>[6x]MFSKFFIERPVFASVVAIIISLAGAIGLTNLPIEQYPSLTPPTVKVSATYTGADAQTIASTVASPIEDAINGADNMIYMDSTSSSSGTMSLTVYFDIGTDPDQATIDVNNRISAATAKMPDAVKKLGVTVRKTSSTTLAAISMYSSDGSMSAVDVYNYITLNVLDELKRVPGVGDANAIGNRNYSLRIWLKPDLLNKFGITATDVISAVNDQNAQYATGKIGEEPVTQKSPYVYSITMQGRLQNPSEFENIILRTNNDGSFLRLKDVADVEIGSQQYSSQGRLNGNDAVPIMINLQSGANALHTAELVQAKMQELSKNFPKGLTYKIPYDTTKFVIESIKEVVKTFVEALILVIIVMYMFLKNFRATLIPMIAVPVSLLGTFAGLYVLGFSINLLTLFALILAIGIVVDDAIIVVENIDRILHENEQISVKDAAIQAMQEVSSPVISIVLVLCAVFVPVSFISGFVGEIQRQFALTLAISVTISGFVALTLTPSLCALFLRRNEGEPFKFVKKFNDFFDWSTSVFSAGVAYILKRTIRFVLIFCIMLGAIFYLYKAVPNSLVPEEDQGLMISIINLPSASALHRTISEVDHISQEVLKTNGVKDAMAMIGFDLFTSSLKENAAAMFIGLQDWKDRNVSADQIIAELNKKFAFDRNASSVFIGLPPIPGLSITGGFEMYVQNKSGKSYDEIQKDVNKLVAAANQRKELSRVRTTLDTTFPQYKLIIDRDKLKHYNLNMQDVFNTMNATIGTYYVNDFSMLGKNFQVNIRAKGDFRNTQDALKNIFVRSNDGKMIPLDSFLTLQRSSGPDDVKRFNLFPAAQVQGQPAPGYTSGQAIEAIAQVAKETLGDDYSIAWSGSAYQEVSSKGTASYAFALGMIFVFLILAAQYERWLIPLAVVTAVPFAVFGSFLLVYLRGFSNDIYFQTGLLLLIGLSAKNAILIVEFAMEERFKKGKGVFEAAVAAAKLRFRPIIMTSLAFTFGVLPMIFATGAGSASRHSLGTGLIGGMIAASTLAIFFVPLFFYLLENFNEWLDKKR

The Cme locus consists of three tandemly linked genes (cmeABC) encoding protein components of the tripartite Cme efflux pump (CmeA, CmeB, and CmeC), where all three components are absolutely required for substrate expulsion. This tripartite system is composed of the CmeB efflux pump, an inner membrane resistance-nodulation-cell division (RND)12 transport protein that contains substrate-binding sites and transduces the electrochemical energy required for pumping drugs out of the cell; the CmeA periplasmic protein, a member of the membrane fusion protein family; and the CmeC outer membrane-associated protein that is integral to the outer membrane. To understand the transport mechanism of the CmeB efflux pump from C. jejuni, we here define the X-ray structures of this membrane protein, which assembles as a trimer. Overall, CmeB adopts the fold of a typical hydrophobe-amphiphile efflux (HAE)-RND-type protein and forms a homotrimer, with its pseudo threefold symmetrical axis positioning perpendicular to the membrane surface. Each subunit of CmeB contains 12 transmembrane helices (TM1-TM12) and a large periplasmic domain created by two extracellular loops between TM1 and TM2, and between TM7 and TM8, respectively.

Two distinct conformations of CmeB with space groups C2 (form I) and P1 (form II) were captured in two different forms of crystals. Surprisingly, in the form II structure, the periplasmic cleft of one of the protomers is open, albeit similar to the conformation of the “binding” state of AcrB. We labeled this conformer as the “binding” form of CmeB. However, the periplasmic clefts of the other two protomers are closed in conformation. One of these two CmeB molecules is more related to the structure of the “extrusion” conformers of the form I structure. Thus, this conformer was classified as the “extrusion” form. Interestingly, the other CmeB molecule of the form II structure displays a distinct conformation, forming a new state that is different from the “extrusion” form. No channel was found in this conformer. This conformation probably represents one of the intermediates that the CmeB pump must go through during the transport cycle. We thus designated this conformation as the “resting” state of the CmeB efflux pump.>[4x]GMNENLENFSTIDLLNELKRRYACLSKPDGRYIFLGAPGSGKGTQSLNLKK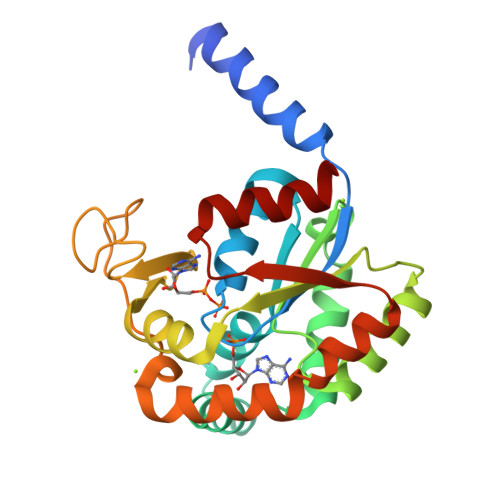SHCYCHLSTGDLLREAAEKKTELGLKIKNIINEGKLVDDQMVLSLVDEKLKTPQCKKGFILDGYPRNVKQAEDLNKLLQKNQTKLDGVFYFNVPDEVLVNRISGRLIHKPSGRIYHKIFNPPKVPFRDDVTNEPLIQREDDNEDVLKKRLTVFKSETSPLISYYKNKNLLINLDATQPANDLEKKISQHIDG> ERRRRAAAVIEEVEQRFSTPTALLRGIADAMVEEMERGLRADPHAPLKMLISYVDNLPTGDEHGLFYALDLGGTNFRVIRVQLGGREKRVVSQQYEEVA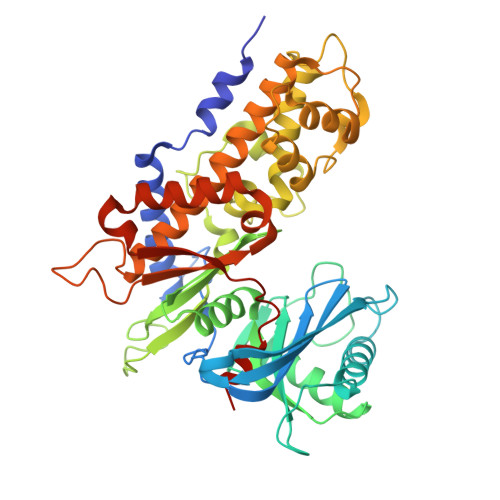IPPHLMVGTSMELFDFIAAELESFVKTEGEDFHLPEGRQRELGFTFSFPVHQTSISSGTLIKWTKGFSINGTVGEDVVAELSRAMERQGLDMKVTALVNDTVGTLAGGRYVDNDVAAAVILGTGTNAAYVEHANAIPKWTGLLPRSGNMVINMEWGNFKSERLPRSDYDNALDFESLNPGEQIYEKMISGMYLGEIVRRILLKLAHDASLFGDVVPTKLEQRFILRTPDMSAMHHDTSHDLKHLGAKLKDILGVADTSLEARYITLHVCDLVAERGARLAAAGIYGILKKLGRDRVPSDGSQKQRTVIALDGGLYEHYKKFRTCLEATLADLLGEEAASSVVVKLANDGSGIGAALLAASHSQYASVE> MSQPQSSQVTKRGLTDPERAAIIAAAVPDHALDTQRKYHYFIQPRWKRLSEYEQLSCYAQPNPDWIAGGLDWGDWTQKFHGGRPSWGNE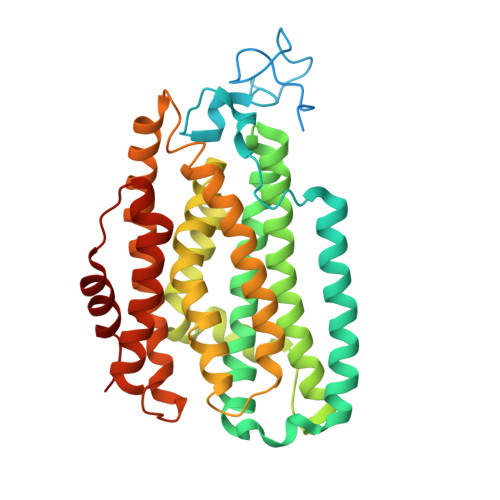STELRTTDWYRHRDPARRWHAPYVKDKSEEARYTQRFLAAYSSEGSIRTIDAYWRDEILNKYYGALLYNEYGLFNAHSSVGRDCLSDTIRQSATFAGLDKVDNAQMIQMERLFIAKLVPGFDASTDVPKKIWTTDPIYAGARGAVEEIWQGIQDWNEILWAGHAVYDATFGQFARREFFQRLATVYGDTLTPFFTAQSQTYFQTTRGAIEDLFVYCLANDPEFGAHNRTFLNAWTEHYLARSVTALKDFVGIYAKVEKVAGATDRAGVSEALQRVFGDWKVDYADKIGFNIDVDQKVDAVLAGFKN~{N}-[1-[[4-(5-oxidanylidene-3-phenyl-6~{H}-1,6-naphthyridin-2-yl)phenyl]methyl]piperidin-4-yl]-3-(propanoylamino)benzamide | C36 H35 N5 O3 | 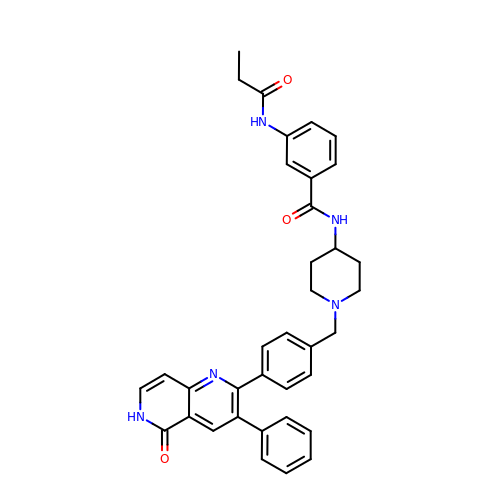IWMRYSJODDURNY-UHFFFAOYSA-N>[6x]LDGRPLAAAGIVVTGDKAVNIYTSSQTGSIIIKLLPNMPKDKEACAKAPLEAYNRTLTTLLTPL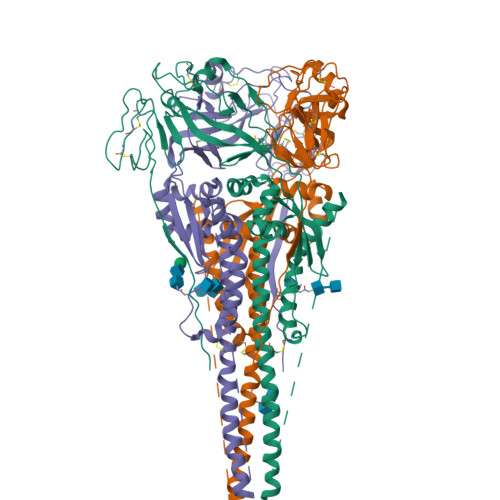GDSIRRIQESVTTSGGGKQGRLIGAIIGGVALGVATAAQITAASALIQANQNAANILRLKESIAATNEAVHEVTNGLSQLAVAVGKMQQFVNDQFNKTAQELDCIKITQQVGVELNLYLTELTTVFGPQITSPALTQLTIQALYNLAGGNMDYLLTKLGVGNNQLSSLISSGLITGNPILYDSQTQLLGIQVTLPSVGNLNNMRATYLETLSVSTTKGFASALVPKVVTQVGSVIEELDTSYCIETDLDLYCTRIVTFPMSPGIYSCLSGNTSACMYSKTEGALTTPYMTLKGSVIANCKMTTCRCADPPGIISQNYGEAVSLIDRQSCNILSLDGITLRLSGEFDATYQKNISIQDSQVIVTGNLDISTELGNVNNSISNALDKLEESNSKLDKVNVKLTSTSSREQKLISEEDLN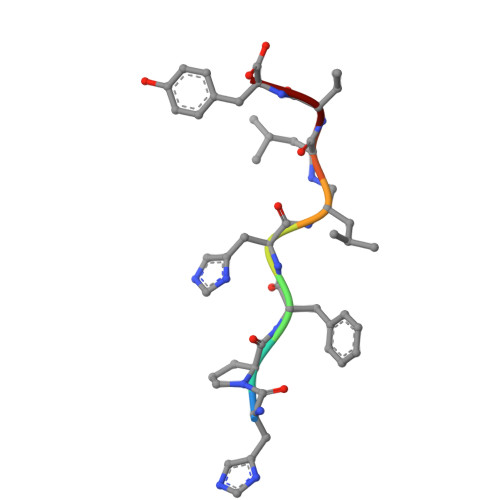> HPFHLLVY> MTDNHIDVLINGCGIGGAMLAYLLGRQGHRVVVVEQARRERAINGADLLKPAGIRVVEAAGLLAEVTRRGGRVRHELEVYHDGELLRYFNYSSVDARGYFILMPCESLRRLVLEKIDGE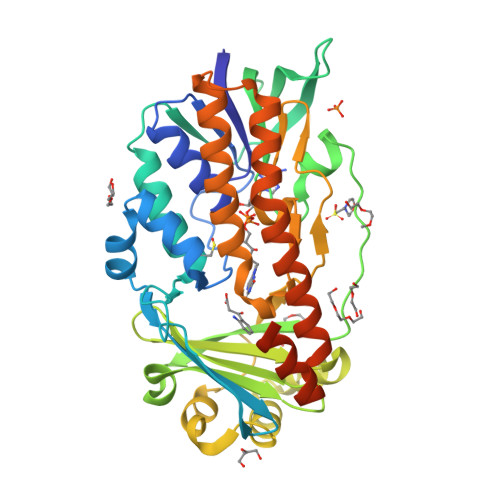ATVEMLFETRIEAVQRDERHAIDQVRLNDGRVLRPRVVVGADGIASYVRRRLLDIDVERRPYPSPMLVGTFALAPCVAERNRLYVDSQGGLAYFYPIGFDRARLVVSFPREEARELMADTRGESLRRRLQRFVGDESAEAIAAVTGTSRFKGIPIGYLNLDRYWADNVAMLGDAIHNVHPITGQGMNLAIEDASALADALDLALRDACALEDALAGYQAERFPVNQAIVSYGHALATSLEDRQRFAGVFDTALQGSSRTPEALGGERSYQPVRSPAPLG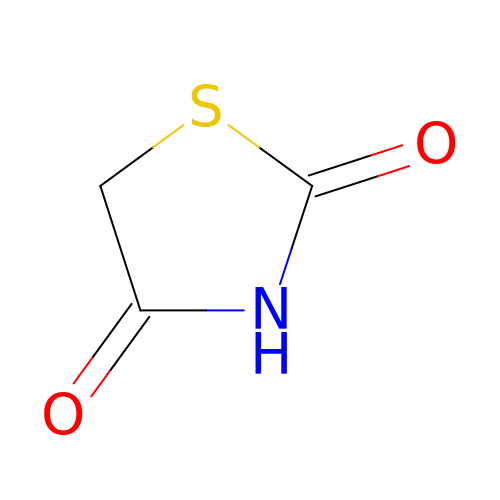1,3-thiazolidine-2,4-dione | C3 H3 N O2 S | ZOBPZXTWZATXDG-UHFFFAOYSA-N>GHMTASPRAPHQEHVLGEPTLEGLAHYIREKNVRRILVLVGAGASVAAGIPDFRSPDTGIYANLGKYNLEDPTDAFSLTLLREKPEIFYSIARELNLWPGHFQPTAVHHFIRLLQDEGRLLRCCTQNIDGLEKAAGVSPELLVEAHGSFAAAACIECHTPFSIEQNYLEAMSGTVSRCSTCGGIVKPNVVFFGENLPDAFFDALHHDAPIAELVIIIGTSMQVHPFALLPCVVPKSVPRVVMNRERVGGLLFRFASTSSSSDGYGQYGDYHAHPDVCRDVLFRGDCQENVVTLAEYLGLSEALAKRMRLSDAAPATAQRAPNET[2x];>[2x]KKGQSTSRHKKLMFKTEG

The proteins belonging to the Silent Information Regulator 2 (SIR2) family, also known as Sirtuins, are classified as class III HDAC proteins due to their dependency on NAD+ to deacetylate lysine residues of histones and non-histone substrates. In Leishmania, cytosolic SIR2rp1 presents NAD+-dependent deacetylase and ADP-ribosyltransferase activities unrelated to epigenetic silencing. While single knockouts were readily obtainable, double deletion of the Sir2rp1 alleles in L. infantum was only possible after the rescue by an episomal copy of the gene, suggesting an essential role for parasite survival. Here we describe the first high-resolution crystal structure of Leishmania infantum SIR2rp1.

Deleting 51 residues from a proteolytically-sensitive region connecting the β8 and β9 strands of the catalytic core led to the crystallization and structural resolution of Leishmania infantum SIR2rp1. Crystals suitable for X-ray diffraction could be obtained only with LiSIR2rp1(ΔP253-E303) mutant, uniquely in the presence of the p53 peptide substrate. Crystals belonged to the P21 space group and contained two LiSIR2rp1(ΔP253-E303) /p53 complexes per asymmetric unit. In addition to a small number of residues missing at both N- and C- terminal ends of the protein (N-ter M1-R6 and C-ter A371-T373 are missing in both monomers), region R52-P70 could not be modeled in monomer B. Moreover, additionally to region P253-E303 removed from the recombinant protein, electron density was missing for residues A304 to P323 in both monomers, suggesting potential flexibility of this region. The two protein monomers of the asymmetric unit are highly similar (rmsd of 0.4Å for all Cα atoms) with a typical sirtuin two-domain structure —a large Rossman-fold domain (pink) and a smaller zinc-binding domain (turquoise). The zinc-binding domain comprises a two-stranded antiparallel β-sheet with four α-helices and includes a Zn2+ ion coordinated by four strictly conserved cysteines (Cys152, 155, 176 and 179). The p53 peptide backbone forms an anti-parallel β-sheet like interaction termed the β-staple, with main chain residues 191 and 192 of the small domain and residue 222 of the large domain. The acetylated side chain of lysine 382 inserts into a hydrophobic tunnel delineated by Val 188 and Val 221. Deeper, the Nζ of the acetylated lysine forms a hydrogen bond with the carbonyl group of Val 188 main chain, and the acetyl group is trapped between Phe 74, His 144, Phe 189 and Phe 190. With similarity to that observed with human and yeast SIR2 homologues, structural comparisons of LiSIR2rp1(ΔP253-E303) complexed with p53 peptide with apo ScHst2, shows a rigid rotation of the Leishmania small zinc-binding domain towards the large domain (≈10°), closing the LiSIR2rp1 binding site.4-chloro-N-[(1R)-1-[1-ethyl-6-(trifluoromethyl)benzimidazol-2-yl]ethyl]benzenesulfonamide | C18 H17 Cl 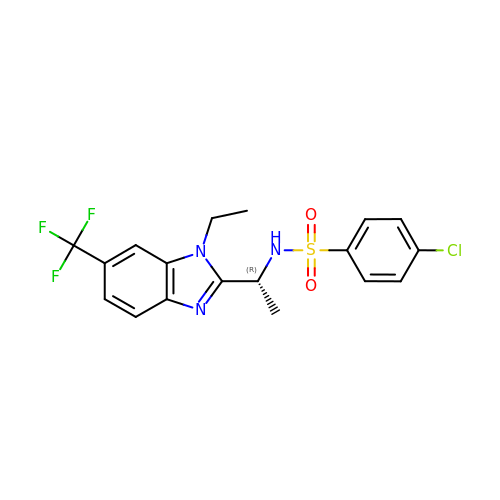F3 N3 O2 S | GZEBDYPIIBQKLB-LLVKDONJSA-N> MLRHTSRNNALHAFVRSPHYRTIPSAGPNGIVVNRDMLVHQFRDFYKTLQHCSLVDKVHLMSERPSVEALRVADQMVSIGATFLEMPLTGMEHRATEFMESMRYVRGAGGPSTLASYLQDTENCRCNSGDVVCLPNGIAVGHGPRTNAVAHTTLKQLFEVKDDQFSFDVFTLEQEGDAPPLGDYFGFAGSNVLLTWKDEHGLLAVDQYQQKQPHTEMNVVYLEPGCHFLSFYGVDHTIDVLVQKGYERSMDSIAAA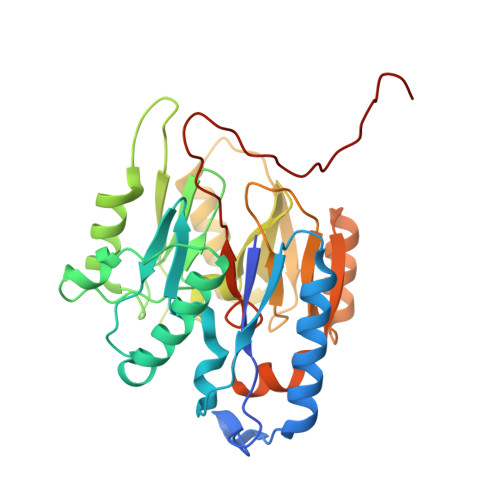GLNPIPVQWSEMDKLGISMRAAVLPLKFFKANVGGMLSRNKSRGARWQTHQLQK1-(2-aminopyridin-4-yl)-3-[(3S)-5-{4-[(E)-(ethoxyimino)methyl]phenoxy}-3-methylpentyl]imidazolidin-2-one 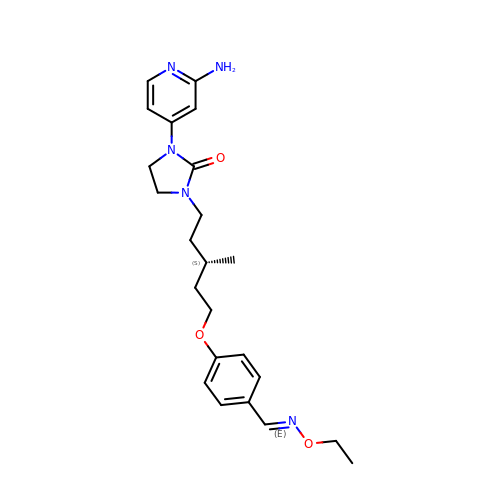| C23 H31 N5 O3 | SRJKGDFZRYDLKM-WYZSWBMLSA-N>GPAVGSCVVCHSQTSLRCGTCIRRPFLCCKCCYDHVIATPHKMVLSVSPYVCNAPGCGVSDVTKLYLGGMSYFCVDHRPVCSFPLCANGLVFGLYKNMCTGSPSIVEFNRLATCDWTESGDYTLANTTTEPLKLFAAETLRATEEASKQSYAIATIKEIVGERQLLLVWEAGKSKPPLNRNYVFTGYHITKNSKVQLGEYIFERIDYSDAVSYKSSTTYKLTVGDIFVLTSHSVATLTAPTIVNQERYVKITGLYPTITVPEEFASHVANFQKSGYSKYVTVQGPPGTGKSHFAIGLAIYYPTARVVYTACSHAAVDALCEKAFKYLNIAKCSRIIPAKARVECYDRFKVNETNSQYLFSTINALPETSADILVVDEVSMCTNYDLSIINARIKAKHIVYVGDPAQLPAPRTLLTRGTLEPENFNSVTRLMCNLGPDIFLSMCYRCPKEIVSTVSALVYNNKLLAKKELSGQCFKILYKGNVTHDASSAINRPQLTFVKNFITANPAWSKAVFISPYNSQNAVSRSMLGLTTQTVDSSQGSEYQYVIFCQTADTAHANNINRFNVAITRAQKGILCVMTSQALFESLEFTELSFTNYKLQ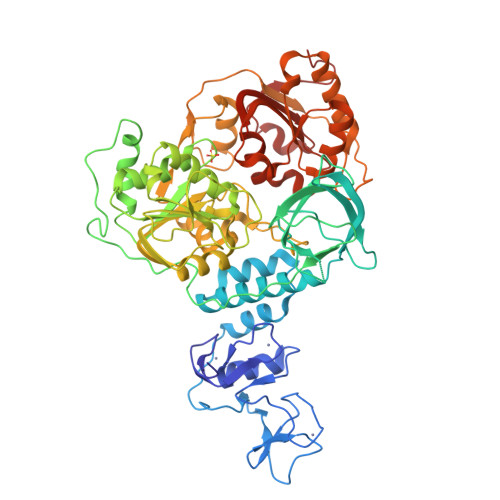[2x]ethyl 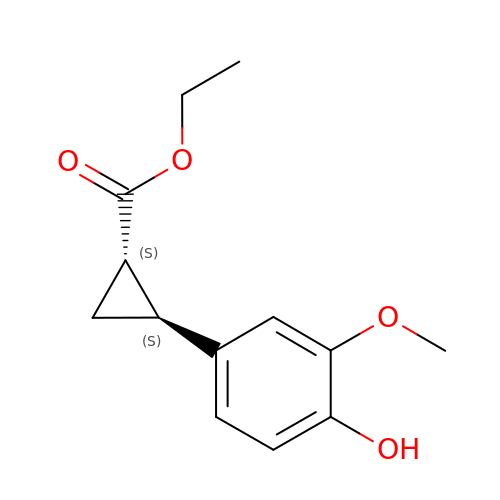(1S,2S)-2-(4-hydroxy-3-methoxyphenyl)cyclopropanecarboxylate | C13 H16 O4 | QZLUEKVALMNAEZ-ZJUUUORDSA-N>MEPKVAELKQKIEDTLCPFGFEVYPFQVAWYNELLPPAFHLPLPGPTMAFLVLSTPAMFDRALKPF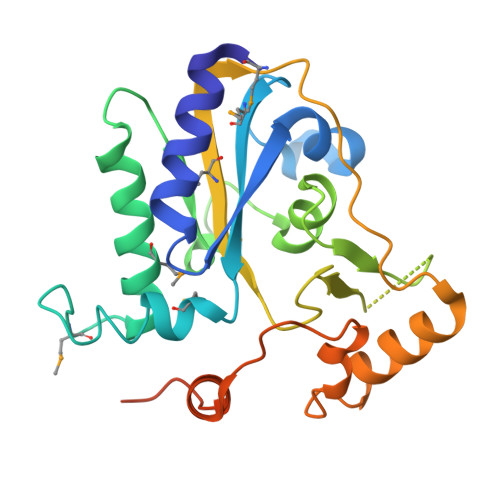LQSCHLRMLTDPVDQCMAYHLGRVRESLPELQIEIIADYEMHPNRRPKILAQTAAHVAGAAYYYQRQDVEADPWGNQRISGVCIHPRFGGWFAIRGVMLLPGIEVPDLPPRKPHDCVPTRADRIALLEGFNFHWRDWTYRDAVTPQERYSEEQKAYFSTPPAQRLALLGLAQPSEKPSLEHHHHHH[2x]>[3x]MTSAEMTSPNNNSEHQAIAKMRTMIEGFDDISHGGLPIGRSTLVSGTSGTGKTLFSIQFLYNGIIEFDEPGVFVTFEETPQDIIKNARSFGWDLAKLVDEGKLFILDASPDPEGQEVVGGFDLSALIERINYAIQKYRARRVSIDSVTSVFQQYDASSVVRRELFRLVA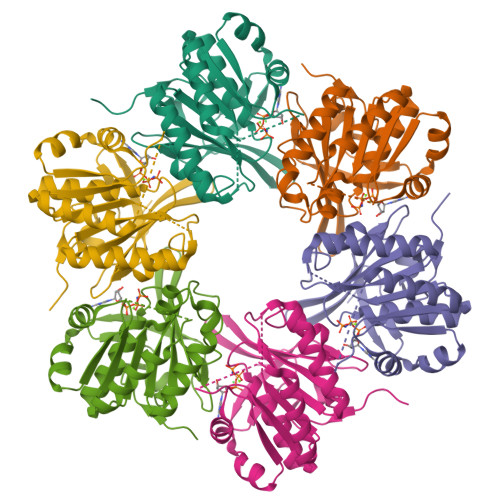RLKQIGATTVMTTERIEEYGPIARYGVEEFVSDNVVILRNVLEGERRRRTLEILKLRGTSHMKGEYPFTITDHGINIFPLGAMR>SNAMNASAVETIYESTEDKAALTSVVD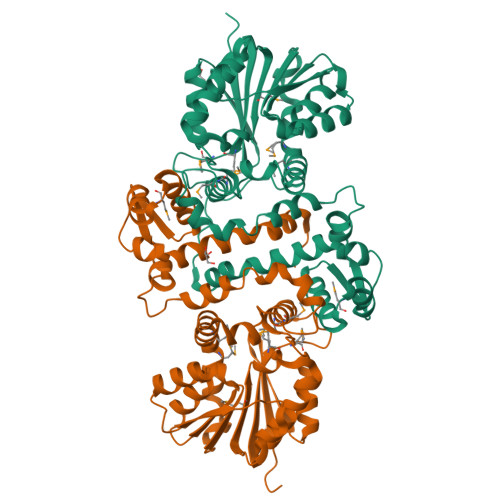LVKLSDQYRQSAILHYAVADKLFDLTQTGRTPAEVAASFGMVEGKAAILLHALAALGLLTKEGDAFRNTALTERYLTTTSADYIGPIVEHQYLQWDNWPRLGEILRSEKPLAFQQESRFAHDTRARDAFNDAMVRLSQPMVDVVSELGVFARARTVIDLAGGHGTYLAQVLRRHPQLTGQIWDLPTTRDAARKTIHAHDLGGRVEFFEKNLLDARNFEGGAADVVMLNDCLHYFDAREAREVIGHAAGLVKPGGALLILTMTMNDDRVTPALSADFSLHMMVNTNHGELHPTPWIAGVVRDAGLAVGERSIGRYTLLIGQRSSGE[2x]>AEPVYPDQLRLFSLGQGVCGDKYRPVNREEAQSVKSNIVGMMGQWQISGLANGWVIMGPGYNGEIKPGTASNTWCYPTNPVTGEIPTLSALDIPDGDEVDVQWRLVHDSANFIKPTSYLAHYLGYAWVGGNHSQYVGEDMDVTRDGDGWVIRGNNDGGCDGYRCGDKTAIKVSNFAYNLDPDSFKHGDVTQSDRQLVKTVVGWAVNDSDTPQSGYDVTLRYDTATNWSKTNTYGLSEAVTTKNKFKWPLVGETELSIEIAANQSWASQNGGSTTTSLSQSVRPTVPARSKIPVKIELYKADISYPYEFKADVSYDLTLSGFLRWGGNAWYTHPDNRPNWNHTFVIGPYKDKASSIRYQWDKRYIPGEVKWWDWNWTI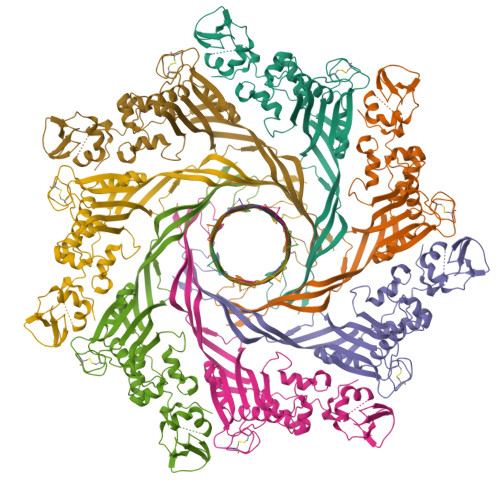QQNGLSTMQNNLARVLRPVRAGITGDFSAESQFAGNIEIGAPVPLAA[7x]>MYAYNGKLLDVDLTREKVKEVELSEDVLKKFYGGRGLGTYILWKELGEKWEKVDPLGEENLLLILTGPLTGYYPGMKTSIVSKSPESNGVVGSVLSSELGLELKAAGYDGIIIRGKAKSPVYLFIHNDTVEIRDATKYWGMGGIELYKTLLKEVHEEIRKKEKLKGVPKEPAMIYIGKGGENKVRFAAIMTKLMHAAGYGGYGAVMGSKNLKAVIAKGSGPLPEVYDKEKMKVLLREFWKELFSMTTFREWGTGAGGYSVGHDRSSEPIRNWQEEYHDNEEISVVNFENRTWIKKYWADYGCPVNCMKISYLRYGPYKGSISDAPDYELQAYMGTNLGIFEPEKIVYLSYLVDELGLDGINTGNILGFAAELYQRGILTKEDLGFELNWGDEKAFAKLLHLIVEKEGIGKILAEGTYRAALKISEIKGIDVTKYAVHVKGIAVGAHGIRSELDYTKDISYAVSVQGGDHTSTAALPAKGYTGELVEAFYDSAVICNFVTKPGFEKIIEFGNALSGFNITPEQWLNEIGLRIIHLQRILLLLGGPDVYWDPRKDDDNPPRFYEPLPSGPVKGKAPNREDIKAKVKQYYEEIGYDEHGIPKEEVLEELGIGEAKREVKRIKKRLNL[2x];>AIWILITPDKCSGCRLCEVTCSLEHEGIIWPEASRIRVFELFPGINVPHTCVQCPDYPCVNACPTNALSVDEKTGAVVVNEEKCITCGACVLACPGKVPRIPAGKGSVVICDLCGGNPKCVEICHEAGHDALKIVTGNYRPIYRTFAKDPQEKSLDIARKVFGEDF[2x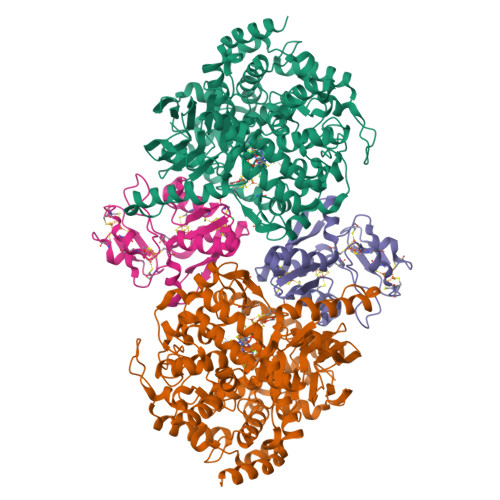]> GAMGMALKKEGPEFDHDDEVLLLEPGIMLDESSADEQPSPRATPKATTSFSSKQHKHIDYTR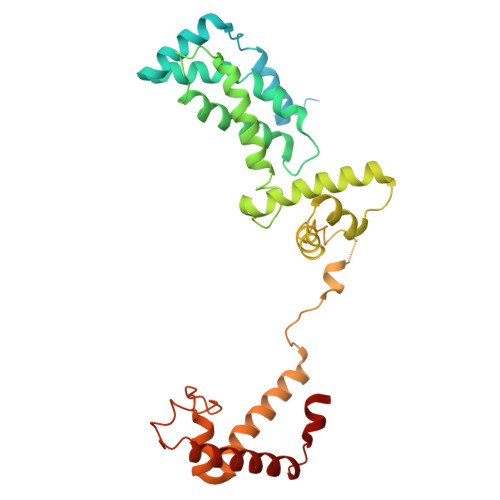ALDATQLYLNEIGFSPLLTPEEEVHFARLAQKGDPAGRKRMIESNLRLVVKIARRYVNRGLSLLDLIEEGNLGLIRAVEKFDPERGFRFSTYATWWIRQTIERAIMNQTRTIRLPIHVVKELNVYLRAARELTHKLDHEPSPEEIANLLEKPVAEVKRMLGLNERVTSVDVSLGPDSDKTLLDTLTDDRPTDPCELLQDDDLSESIDQWLTELTDKQREVVIRRFGLRGHESSTLEEVGQEIGLTRERVRQIQVEALKRLREILEKNGLSSDALFQ6-carbamimidoyl-N-phenyl-4-(pyrimidin-2-ylamino)naphthalene-2-carboxamide | C22 H18 N6 O | 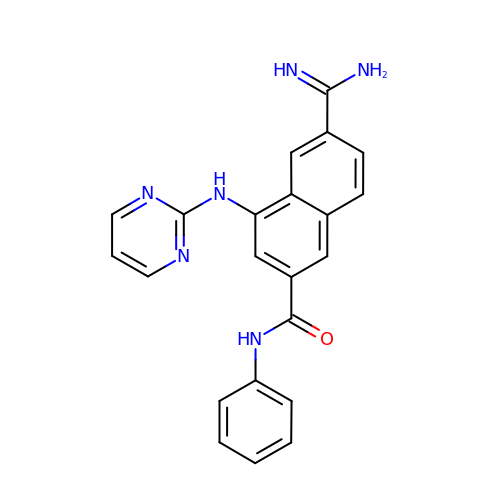MMMVHDBARFPCLX-UHFFFAOYSA-N>MGGSHHHHHHGDDDDKMVEFPEGFVWGAATSGPQTEGNFHKQHQNVFDYWFATEPEQFDAGVGPDTASNFYNDYDHDLALMAQAGVQGLRTSIQWTRLIDDFETASLNADGVAFYNHVIDSMLAHHITPYINLHHFDLPVALYDKYHGWESKHVVELFVKFAEQCFKLFGDRVDHWYTFNEPKVVVDGQYLYGWHYPQVINGPKAVQVAYNMNLASAKTVARFHELSVRPEQQIGIILNLTPAYAASDDPADLAAAEFAELWSNNLFLDPAVLGHFPEKLVERLTMDGVLWDATPTELAIIAANPVDSLGVNYYHPFRVQRPDISPKSLQPWMPDIYF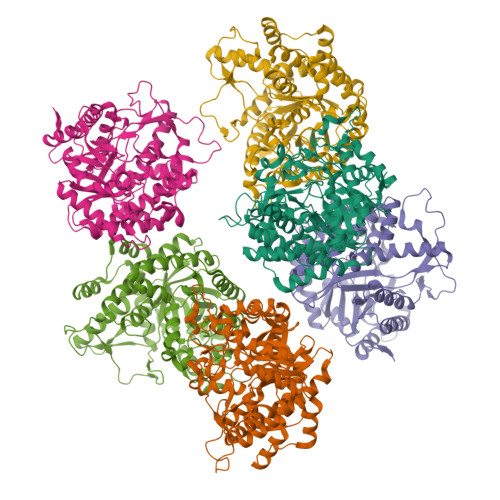KEYDMPGRMMNVDRGWEIYPQAMTDIARNIQKNYGNIPWMISENGMGVAGEERFLDKQGVVQDDYRIDFMKEHLTALAKGIAAGSNCQGYFVWSGIDCWSWNHAYHNRYGLIRNDIHTQTKTLKKSAKWFAELGERNGF[6x]>LKCHNTQLPFIYKTCPEGKNLCFKATLKKFPLKFPVKRGCADNCPKNSALLKY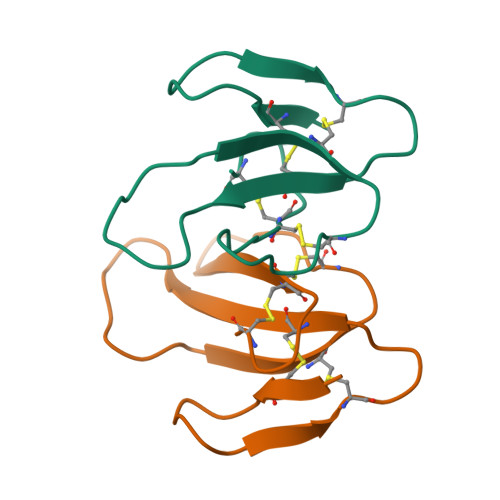VCCSTDKCN[2x]>MSNCQYKIYPPLGIARVGNGPAIKPLSLSTPEVPWAHLYDTNVQYLVTQQELEQLLEEAFGGNVINEISQIKTKLDERKAEKFKQEEIETITGLLGLSHLVPQQQLSRSLDNLELKSTKDSDDI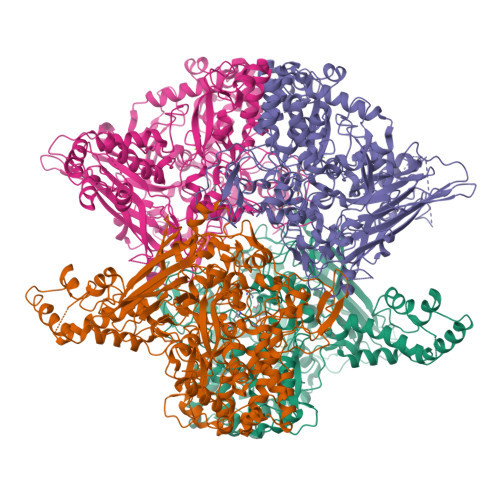VQQIKGALLKVLSDHYLHAVKKQAQNFYIYKCDEQGNPVEKLKLTDGDKVTWRVEVANKKSFWYDYNNALDLSLHTQGSGNLSKNVSKHRLAPAMTAKRRNPNVITNSLRKQLVISSQGSVSSDNNTQVPLRGKFPANEPDTNNRLSDLLNLQERHNVLQGSIECDNEGVLRFYAGNGISQALSPSSLNTDFADNSNWFDDICDGRVTAVVELKNGDTFEIQDEQSSAWVATTPPDYAPQIEPIVTMYDMVSGAALKEQDLDNLTTQFSDVFPILYRLYRMQWVNQADFTDNAVNTQIRELNSELGFAQLLDNSASAKSLREGIFNQFRNPLFDQDIDVDDPGQSSNEWVSNSRIIPSKDETNIAAKPATSSLKLPFYPNDGIDYPGSPVQWFAIPPFMYQHLQNWAAGDFSVTQVEKESANTIEELGLFYSEQFKNSPNSALLCARGALDALYGGGFHPGVELTWPMRHNLIYSQNDYVSSVTPEINLLGLREFRLKQDLQGLNSPNMYQDFGHVIAVDNVTASIDPNSDAAWLWRSTPGDLTKWMGIPWQSNAASCQAVYTPEDFPIPSWWAANLPVHVLPLARYNKFKDSQSADLPEINGMTHSIAQGMSEETFEHLRLEQFSQRLDWLHTADLGFVGYHAEGGYTNGLIQMVSQWKNMAMVMARPVENPGSSGIPNVVYVAYSQADKD[4x]>[2x]MNELIKYAKELVRSAGKTLKSAAMFAKVLTPNDDSG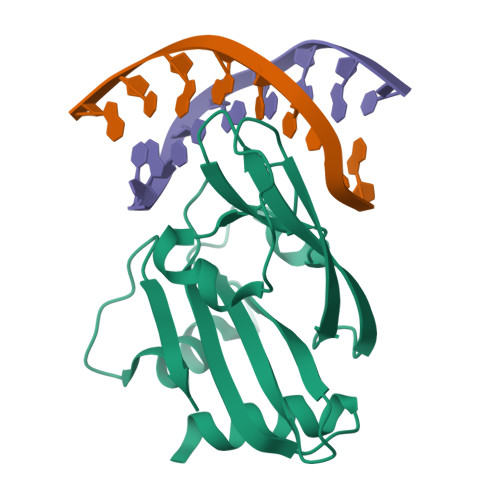RHGVLVPTEAYSFFPDMPISDPSQNATSNFPAFDSLSKTHKTLAYKYYERYPERRITRMHGLLNERNYDPRLTIFLFARHTDGSSGYYFDCANSGSGGRFEVLFALCFGEAISPKAGLFVVRPIDSPALEGHHHHHHDSPALEGHHHHHH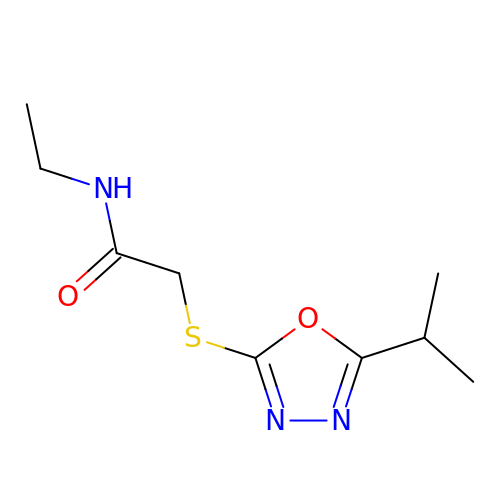N-ethyl-2-{[5-(propan-2-yl)-1,3,4-oxadiazol-2-yl]sulfanyl}acetamide | C9 H15 N3 O2 S | DWIDCIXKOJCTSJ-UHFFFAOYSA-N> GHMKV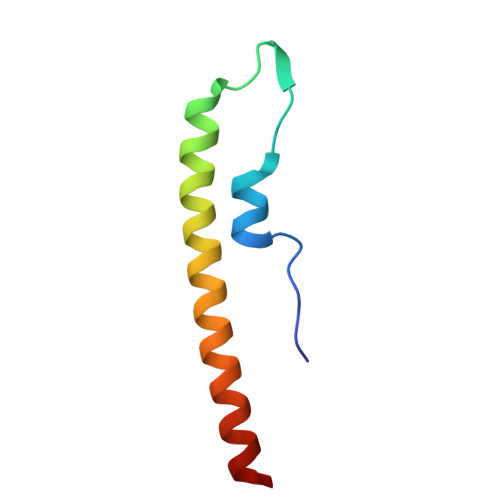KLSAKEILEKEFKTGVRGYKQEDVDEFLDMIIKDYETFHQEIEELQQENLQLKKQLEE>MKDKVYKRPVSILVVIYAQDTKRVLML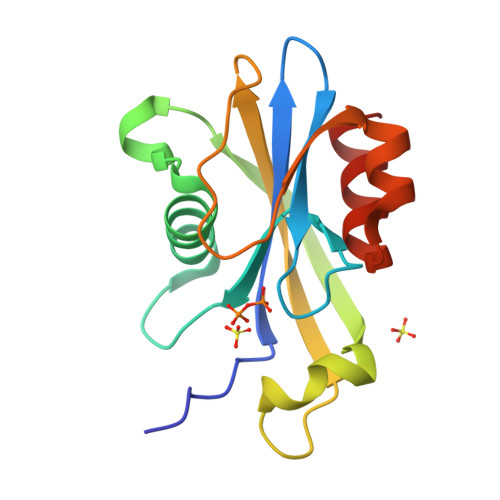QRRDDPDFWQSVTGSVEEGETAPQAAMREVKEEVTIDVVAEQLTLIDCQRTVEFEIFSHLRHRYAPGVTRNTESWFCLALPHERQIVFTEHLAYKWLDAPAAAALTKSWSNRQAIEQFVINAA[4x]> APGQKECDNALRQLETVRELLENPVQPINDMSYFGCLDSVMENSKVLGEAMTGISQNAKNGNLPEFGDAIATAS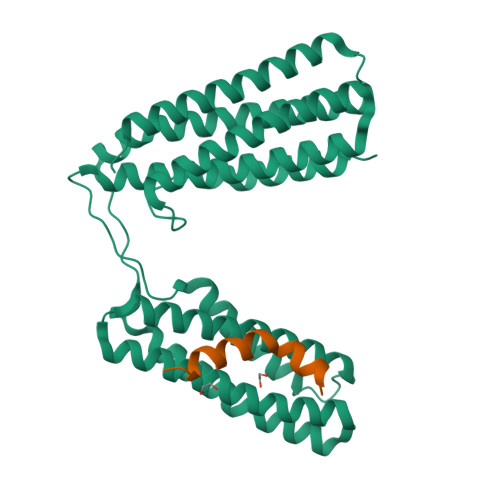KALCGFTEAAAQAAYLVGVSDPNSQAGQQGLVEPTQFARANQAIQMACQSLGEPGCTQAQVLSAATIVAKHTSALCNSCRLASARTANPTAKRQFVQSAKEVANSTANLVKTIKALDGDFTEENRAQCRAATAPLLEAVDNLSAFASNPEFSSVPAQISPEGRAAMEPIVISAKTMLESAGGLIQTARALAVNPRDPPRWSVLAGHSRTVSDSIKKLITSMRDKAPG;> NEDIDQMFSTLLGEMDLLTQS> SMAAG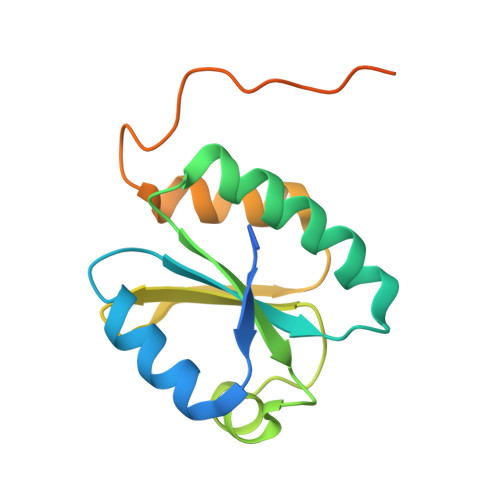AAEAAVAAVEEVGSAGQFEELLRLKAKSLLVVHFWAPWAPQCAQMNEVMAELAKELPQVSFVKLEAEGVPEVSEKYEISSVPTFLFFKNSQKIDRLDGAHAPELTKKVQRHASSGSFLPSAKVKVDTDPNSSSVDKLAAALEHHHHHH>HCRLDKSNFQQPYITNRTFMLAKEASLADQNTDVRLIGEKLFHGVSMSERCYLMKQVLQFTLEEVLFPQSDRFQPYMQEVVPFLARLSNRLSTCHIEGDDLHIQRNVQKLKDTVKKLGESGEIKAIGELDLLFMSLRNACI[2x];>[2x]APEDPSDLLQHVKFQSSNFENILTWDSGPEGTPDTVYSIEYKTYGERDWVAKKGCQRITRKSCDLTVETGDLQELYYARVTAVSAGGRSATKMTDRFSSLQHTTLKPPDVTCISKVRSIQM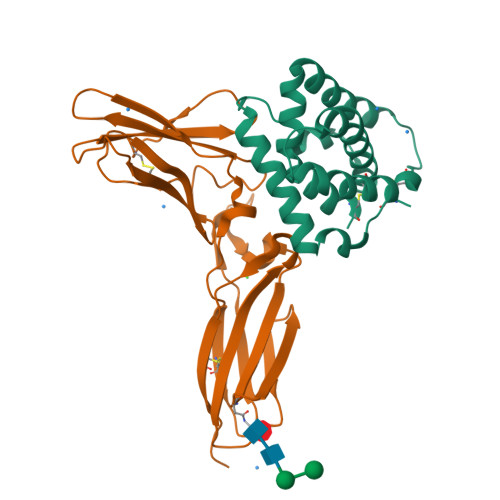IVHPTPTPIRAGDGHRLTLEDIFHDLFYHLELQVNRTYQMHLGGKQREYEFFGLTPDTEFLGTIMICVPTWAKESAPYMCRVKTLPDRT> 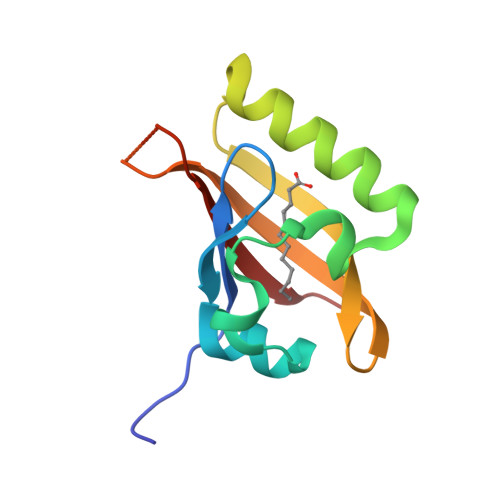QVVSEANSVIVILDRHGNIQRFNRLSEEYTGLKEQEVIGQNVFTLFMSPAEASASRRNVTGFFRNGSSYEVERWIKTRKGQRLFLFRNKFVHSGSGRNEIFLICSGTDIT> MGSDKIHHHHHHENLYFQGMSRKVILTCAVTGNAPFNPKHPSMPITPAQIADACVEAAKAGASVAHIHVRDPKTGGGSRDPVLFKEVVDRVRSSGTDIVLNLTCGLGAFLLPDPEDESKALPESDVVPVAERVKHLEDCLPEIASLDITTGNQVEGKLEFVYLNTTRTLRAMARRF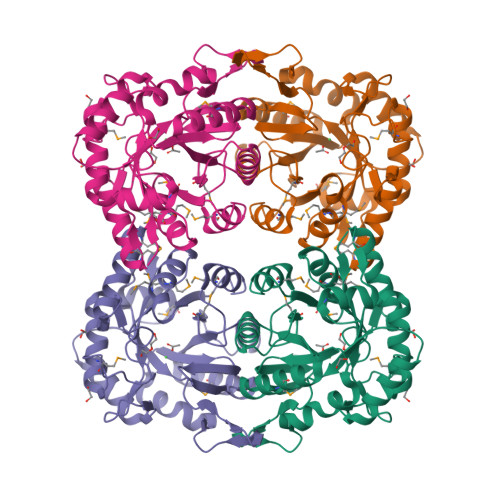QELGIKPELEVFSPGDILFGKQLIEEGLIDGVPLFQMVLGVLWGAPASTETMIYQRNLIPANAQWAAFGIGRDQMPMMAQAALLGGNVRVGLEDNLYLSRGVFATNGQLVERARTVIEHLGMSVATPDEARDIMGLSRPA>[2x]GPLGSMRMTWNFHQYYTNRNDGLM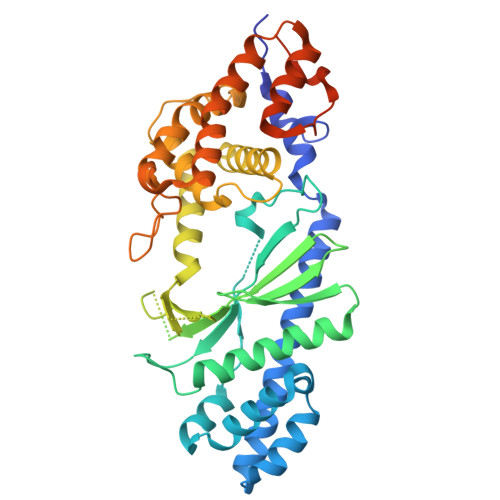GKLVLTDEEKNNLKALRKIIRLRTRDVFEEAKGIAKAVKKSALTFEIIQEKVSTTQIKHLSDSEQREVAKLIYEMDDDARDEFLGLTPRFWTQGSFQYDTLNRPFQPGQEMNINDGTYMPMPIFESEPKIGHSLLILLVDASLKSLVAENHGWKFEAKQTCGRIKIEAEKTHIDVPMYAIPKDEFQKKQIALEANRSFVKGAIFESYVADSITDDSETYELDSENVNLALREGDRKWINSDPKIVEDWFNDSCIRIGKHLRKVCRFMKAWRDAQWDVGGPSSISLMAATVNILDSVAHDASDLGETMKIIAKHLPSEFARGVESPDSTDEKPLFPPSYKHGPREMDIMSKLERLPEILSSAESADSKSEALKKINMAFGNRVTNSELIVLAKALPAFAQEPSSASKPEKISSTMVSGHHHHHH> MALERQEVKNPTGIVTDIAPADLPLEKWSFGNNVRFKNGKAQKALGHTPIFDTAQAPILDMFPFIRNNIPYWLLCGEQRMYLADGTTVVDVSPGGHSASVTSRWSSGSFNGVIFANNPSNYPYVLMPQNSGFIPM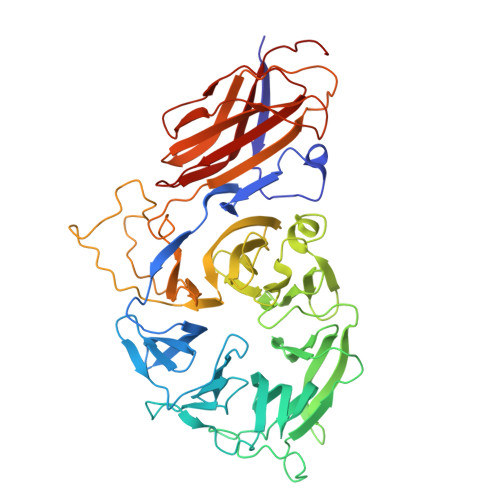PNWPANTFAKRMKSFKNFMIALNVTQNSVEMPQMVWWSTSADAGGIPVSWDPTDPTKDAGQNTLADTNGAIVDGVKLRDSFIIYKEDSVYSMRYIGGLFIFQFQQLFNDVGILGPNCAIEFDGNHFVVGHGDVYVHNGVQKQSVIDAQVRKFFFSDINPDNYQRTFVIADHVNTEMWVCYSSTRSEPGKHCDRAIIWNWKENTWSIRDLPNVLSGAYGIIDPKVSNLWDDDPNPWDTYTSVWGEGSYNPAKSSMIFSSFQDKKLFLFGNNSTFSGQNFVSTLERSDIYLGDDRMMKTVSAIIPHITGNGTCNIWVGNAQVQGSGIRWKGPYPYRIGQDYKIDTKHVGRYIALKFDFSSEGDWYFNGYTIEMAPKAGMR>SNAMSKLPENFLWGGAVAAHQLEGGWQEGGKGISVADVMTAGRHGVAREITAGVLEGKYYPNHEAIDFYHHYKEDVKLFAEMGFKCFRTSIAWTRIFPKGDEAEPNEAGLQFYDDLFDECLKYGIEPVVTLSHFELPYHLVTEYGGFTNRKVIDFFVHFAEVCFRRYKDKVKYWMTFNEINNQANYQEDFAPFTNSGIVYKEGDDREAIMYQAAHYELVASARAVKIGHAINPNLNIGCMVAMCPIYPATCNPKDILMAQKAMQKRYYFADVHVHGFYPEHIFKYWERKAIKVDFTERDKKDLFEGTVDYIGFSYYMSFVIDAHRENNPYYDYLETEDLVKNPYVKASDWDWQIDPQGLRYALNWFTDMYHLPLFIVQNGFGAIDQVEADGMVHDDYRIDYLGAHIKEMIKAVDEDGVELMGYTPWGCIDLVSAGTGEMRKRYGFIYVDKDDEGKGTLKRSPKLSFNWYKEVIASNGDDI[2x]

Specifically, the β-­glycosidic bond of 6′-P-β-glucoside is cleaved by 6-P-β-glucosidase (6PβGlu; EC 3.2.1.86), releasing 6-P-β-glucose (BG6; glycon), an important cellular precursor, and the remaining portion of the given substrate (aglycon). Here, the high-resolution crystal structures of GH1 6-P-β-glucosidases from Lactobacillus plantarum (LpPbg1) and Streptococcus mutans (SmBgl) and their complexes with ligands are reported. 6PβGlu is a single-domain protein that adopts a (β/α)8-barrel (TIM-barrel) structure, which is a typical fold of GH1-family members. The GH1-family enzymes utilize a double-displacement mechanism of catalysis with retention of configuration at the anomeric C atom of the glycon moiety.

Interestingly, the active-site E375Q SmBgl mutant also showed some residual catalytic activity (0.8% of the wild-type enzyme activity detected for gentiobiose).> SNAMPEADRELVSIRRFLKERLQRDYTTLRGYAKERSNVRLLLQRTAEMGESNSLLLLGPRGSGKTTLINSVLADLLPNKSFGENTLIVHLDGNLHTDDRVALKSITVQMQLENAADGKVFGSFAENLAFLLQCLKAGGKHSKSVIFILEEFDLFCAHHNQTLLYNLFDVSQSAQAPICVLGVTCRLDVIELLEKRVKSRFSHRQVFLFPSLRRFEDYVDLCRDLLSLPTGNSLLLAAEKIYNLQNIQSGALYFSRNHFDPGEYGFSPRLRDAWNKQICKVLATQQARSTLQALHDFDISEAYLKNFLFRLVAHLRPQSPHITAEKMAAVGSQFEGDDKIELLCGLSVLELCLIIAIKHHSQIYDRDSFNF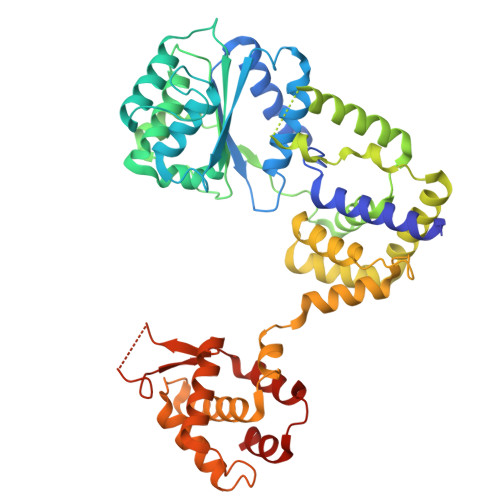EIIYARFSKFAKVSTTMQAVERSIVLKAFEHLRIAELIMPLTGGAGGGVGKVQKEFEMHKLALTYSQIHHCMQRYQALPTEVAQWAQSSLI>MSGGDGRGHNTGAHSTSGNINGGPTGIGVSGGASDGSGWSSENNPWGGGSGSGIHWGGGSGRGNGGGNGNSGGGSGTGGNLSAVAAPVAFGFPALSTPGAGGLAVSISASELSAAIAGIIAKLKKVNLKFTPFGVVLSSLIPSEIAKDDPNMMSKIVTSLPADDITESPVSSLPLDKATVNVNVRVVDDVKDERQNISVVSGVPMSVPVVDAKPTERPGVFTASIPGAPVLNISVNDSTPAVQTLSPGVTNNTDKDVRPAGFTQGGNTRDAVIRFPKDSGHNAVYVSVSDVLSPDQVKQRQDEENRRQQEWDATHPVEAAERNCERARAELNQANEDVARNQERQAKAVQVYNSRKSELDAANKTLADAIAEIKQFNRFAHDPMAGGHRMWQMAGLKAQRAQTDVNNKQAAFDAAAKEKSDADAALSAAQERRKQKENKEKDAKDKCAMESKRNKPGKATGKGKPVGDKWLDDAGKDSGAPIPDRIADKLRDKEFKSFDDFRKAVWEEVSKDPELSKNLNPSNKSSVSKGYSPFTPKNQQVGGRKVYELHHDKPISQGGEVYDMDNIRVTTPKRHIDIHRGK[4x];>[4x]MELKHSISDYTEAEFLQL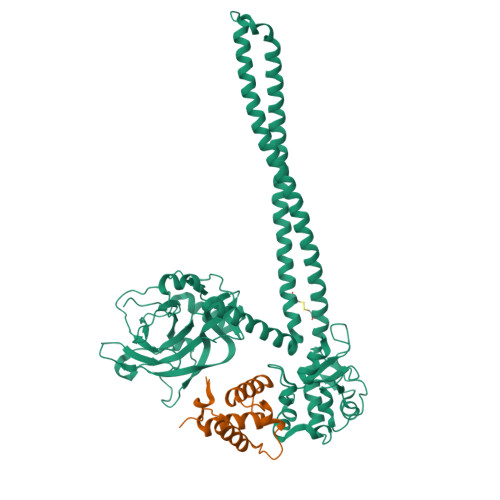VTTICNADTSSEEELVKLVTHFEEMTEHPSGSDLIYYPKEGDDDSPSGIVNTVKQWRAANGKSGFKQGLEHHHHHH> LYPEEILDTHWELWKKTHRKQYNNKVDEISRRLIWEKNLKYISIHNLEASLGVHTYELAMNHLGDMTS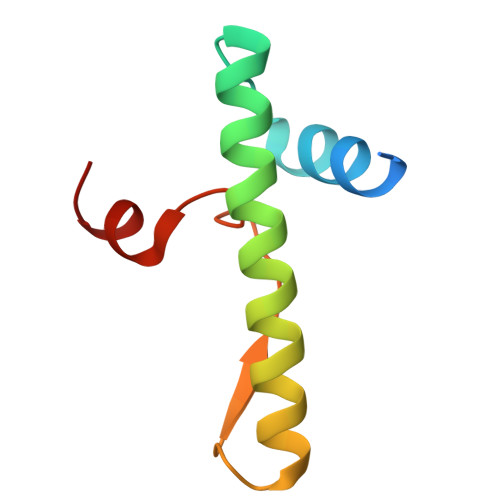EEVVQK>[3x]GSHAVSTQPNPENVAQVTVDPLNDPNSPLAKRSVYFDF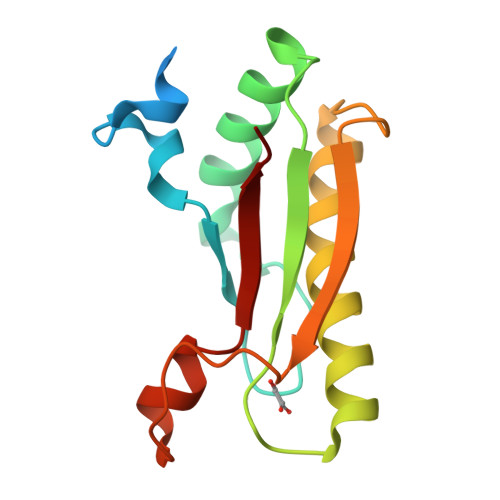DSYSVQDQYQALLQQHAQYLKSHPQRHILIQGNTDERGTSEYNLALGQKRAEAVRRALSLLGVGDAQMEAVSLGKEKPVALGHDEASWAQNRRADLVYQQ>SLRSMVSDSVDEIVDGVSKTTAEVINGRKSIAQYATSLIENNPEPDNVRTIISQPLIKNTFLLVGFGLEKDGSNINNDPSWNPGPTWDPRVRPWYKDAKNAGKLVITAPYADSASGEILVSVATPVKDSATGQFLGSIFYDVSLAELAELVNEVKLFDAGYVFIVSEDGTTIAHPKKEFNGKPMSEFLGESKINVDTHQVIINGKP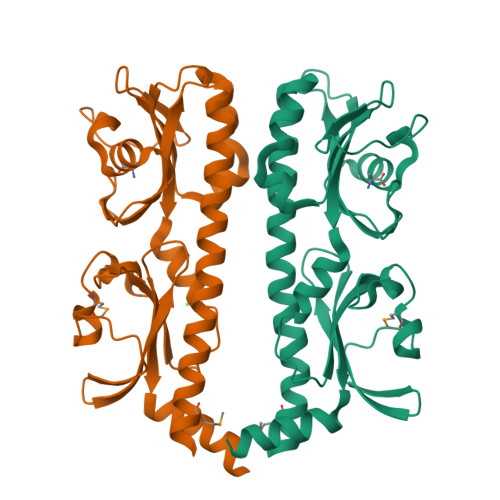YAVSFSDVEGEDWYVGVVIDEEIAYAALDELRRS[2x]>HGYVESPASRSYLCKQGVNVNCGPIQYEPQSVEGIGGFPQLGPSDGQIAGAGHFPALDVQTVDRWKKVTLNGGTN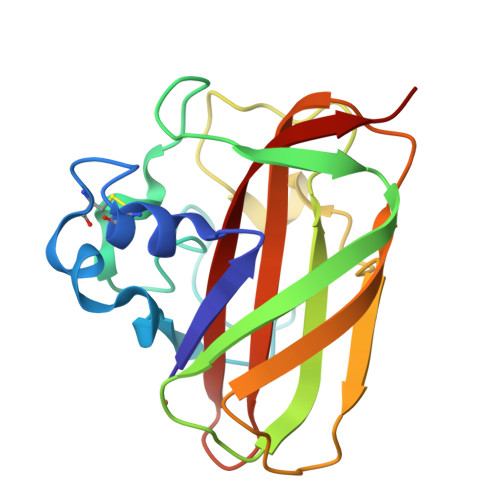TFKWKLTAPHSTKEWKYYITKKGWNPNKPLTRSDLDLVPFYVKNDGGARPGTTVTHEANVPTDRSGYHLILAVWEIADTGNAFYQVIDVNLLNN[4x]Ser/Thr protein phosphatase 1 (PP1) forms a large nuclear holoenzyme (with PNUTS, WDR82, and Tox4) whose emerging role is to regulate transcription. The PP1 nuclear targeting subunit (PNUTS, also known as PPP1R10/p99/FB19/CAT53), which is one of the most abundant regulatory proteins of PP1 in the nucleus, has emerged as an essential regulator of gene expression. Tox4 is predicted to be a largely unstructured member of the DNA-binding high-mobility group box protein family, which has been reported to restrict RNAPII pause release and early elongation, promote late elongation, and facilitate transcriptional reinitiation.

PNUTS adopts a nine α-helical bundle structure consistent with the PNUTSTND solution structures; its structure is most similar to the IWS1/Spn1 protein (DALI Z scores = 13.4–13.8).42 PNUTS helices 5–9 form the TFIIS N-terminal domain (TND), which is a conserved scaffold enriched in transcription factors that mediates binding with TND-interacting motifs (TIMs) and is the domain that exhibits the greatest overlap with IWS1. This domain has previously been shown to bind directly to the MYC TIM (34VQPYF38) in addition to TIMs from other transcription factors (including SPT6 and PAF1).34 Helices 1–4, which pack tightly against the TFIIS domain to form a single compact fold, adopt a distinct α-helical bundle that is not present in other known TFIIS TND-containing proteins. The Tox4CTD adopts a novel conformation, where aa 571–596 form a zinc binding loop in which Tox4 residues Cys572, Cys577, Cys592, and Cys596 coordinate a zinc ion, while residues 597–612 form a long α helix (the Tox4 PNUTS binding helix). The binding interface between Tox4 and PNUTS is extensive, with the Tox4 PNUTS binding helix interacting with PNUTS α helices α1 and α3 via hydrophobic and ionic interactions. The hydrophobic interactions are toward the center of the Tox4-PNUTS interface (Figure 2D; Tox4: W587Tox4, Tyr591Tox4, Val597Tox4, Val598Tox4, Val604Tox4, Phe605Tox4, Trp608Tox4, V609Tox4; PNUTS: Pro8PNUTS, Leu12PNUTS, Leu19PNUTS, Met44PNUTS, Val45PNUTS, Ile53PNUTS, Pro89PNUTS, Leu90PNUTS). Finally, consistent with its nanomolar binding affinity, the complex buries 2,100 Å2 of solvent-accessible surface area. Finally, subsequent isothermal titration calorimetry (ITC) experiments showed that Tox4CTD and PNUTSTND bind tightly, with a KD = 0.3 ± 0.1 nM.

> GHMPIDPKELLKGLDSFLTRDGEVKSVDGIAKIFSLMKEARKMVSRSTYLNIILQTRAPEVLVKFIDVGGYKLLNSWLTYSKTTNNIPLLQQILLTLQHLPLTVDHLKQNNTAKLVKQLSKSSEDEELRKLASVLVSDWMAVIRSQSSTQPAEKDKKKR;> GHMRCVRSGCENPPIVSKDWDNEYCSNECVVKHSRDVFLAWVASRNSNTVVFVK> MLKQPIQAQQLIELLKVHYGIDIHTAQFIQGGADTNAFAYQADSESKSYFIKLKYGYHDEINLSIIRLLHDSGIKEIIFPIHTLEAKLFQQLKHFKIIAYPFIHAPNGFTQNLTGKQWKQLGKVLRQIHETSVPISIQQQLRKEIYSPKWREIVRSFYNQIEFDNSDDKLTAAFKSFFNQNSAAIHRLVDTSEKLSKKIQPDLDKYVLCHSDIHAGNVLVGNEESIYIIDWDEPMLAPKERDLMFIGGGVGNVWNKPHEIQYFYEGYGEINVDKTILSYYRHERIVEDIAVYGQDLLSRNQNNQSRLESFKYFKEMFDPNNVVEIAFATEQLEHHHHHH

For aminoglycosides, a group of antibiotics used to treat serious nosocomial infections, the main mechanism of resistance is via the enzymatic inactivation of the drug by acetyltransferases, nucleotidyltransferases, or phosphotransferases. Among the three types of aminoglycoside-modifying enzymes, aminoglycoside phosphotransferases or kinases (APHs) yield the highest levels of resistance thereby providing a rationale for focusing inhibitor development for these specific resistance factors. Combined, these studies reveal that although members of the APH family share low similarities in sequence and their ligand specificity varies greatly, their overall three-dimensional fold is homologous to each other and to that of ePKs. To further examine the suitability of the CKI-7 scaffold for inhibitor development, we determined the crystal structures of APH(3′)-IIIa and APH(9)-Ia in complex with CKI-7.

APH(9)-Ia is an atypical APH which phosphorylates only one aminoglycoside, spectinomycin, that is distinct from the other aminoglycoside antibiotics. Paralleling the APH(3′)-IIIa result, CKI-7 was found to inhibit APH(9)-Ia (Ki = 159±11 µM) in a competitive fashion with respect to ATP, although 2.5 times less effectively. The CKI-7-bound APH(9)-Ia complex was crystallized in space group P3121 with one molecule per asymmetric unit. This structure has been refined to 2.9 Å and a final Rcryst and Rfree of 0.222 and 0.279, respectively. For APH(9)-Ia, this same loop (residues 28–34) also adopts a different conformation in the APH(9)-Ia-CKI-7 structure compared to the nucleotide-bound state. In fact, the conformation observed is comparable to what is observed for APH(3′)-IIIa, i.e. the tip of loop in the CKI-7-bound APH(9)-Ia also dips into the phosphate-binding area of the nucleotide binding pocket. Intriguingly, despite the conserved nature of this residue, the aromatic side chain of Tyr42 of APH(3′)-IIIa points toward the linker region of the protein whereas the side chain of Phe50 in APH(9)-Ia points in the opposite direction toward the ribose- and phosphate-binding pockets. In APH(9)-Ia, the aminoethyl group of the inhibitor is positioned in the entrance pocket or the solvent-exposed side of the adenine-binding pocket and it points back at itself forming an intramolecular interaction with the equatorial sulfonyl oxygen atom (O2S). The inhibitor also makes a second interaction with the linker region of APH(9)-Ia via the Nβ of the aminoethyl tail and the main chain carbonyl of Ile103. As a result, the orientation and conformation of CKI-7 observed in APH(9)-Ia mirrors what is seen in CK1.>[2x]MGHHHHHHMLHLLEQIRAYCETCWEWQEAHEPGMDQDKNPMPAPVEHQICPAVCVLMKLSFDEEHRHAMNELGGLQAIAELLQVDCEMYGLTNDHYSITLRRYAGMALTNLTFGDVANKATLCSMKGCMRALVAQLKSESEDLQQVIASVLRNLSWRADVNSKKTLREVGSVKALMECALEVKKESTLKSVLSALWNLSAHCTENKADICAVDGALAFLVGT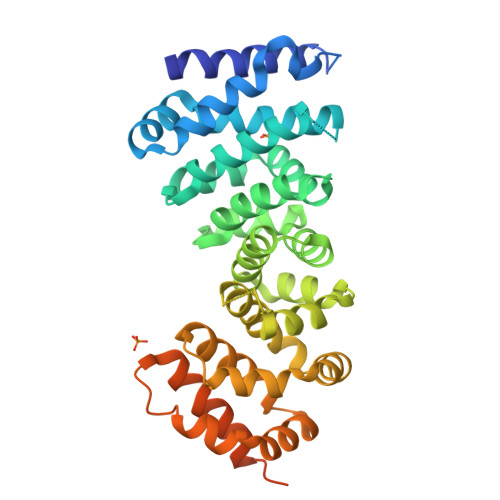LTYRSQTNTLAIIESGGGILRNVSSLIATNEDHRQILRENNCLQTLLQHLKSHSLTIVSNACGTLWNLSARNPKDQEALWDMGAVSMLKNLIHSKHKMIAMGSAAALRNLMANRPAKYKDANIMSPGSSLPSLHVRKQKALEAELDAQHLSETFDN>HYTFPKVWANSGTTADWQYVRRADNWQNNGFVDNVNSQQIRCFQSTHSPAQSTLSVAAGTTITYGAAPSVYHPGPMQFYLARVPDGQDINSWTGEGAVWFKIYHEQPTFGSQLTWSSNGKSSFPVKIPSCIKSGSYLLRAEHIGLHVAQSSGAAQFYISCAQLSITGGGSTEPGANYKVSFPGAYKASDPGILININYPVPTSYKNPGPSVFTC[2x]

An oxidative system was recently discovered in which extracellular flavocytochromes, that is, cellobiose dehydrogenases (CDHs), cooperate with copper-dependent lytic polysaccharide monooxygenases (LPMOs)8910111213 to catalyse redox-mediated glycosidic bond cleavage in crystalline cellulose, hemicelluloses and starch. CDHs are large flavocytochromes containing a haem b-binding cytochrome domain (CYT) connected by a long, flexible linker to a flavin adenine dinucleotide (FAD)-binding dehydrogenase domain (DH). The DH domain oxidizes cellobiose at the C1 position to cellobiono-1,5-lactone with reduction of FAD. The ensuing step involves inter-domain electron transfer (IET) from the reduced FAD to CYT haem b, presumably by single electron-transfer (ET) events, followed by ET from CYT to external electron acceptors such as LPMOs.

NcLPMO9F primarily attacks crystalline cellulose and promotes, in combination with cellulases, faster and more complete surface degradation. The structure of NcLPMO9F demonstrates that this LPMO shares the essential features of fungal LPMOs, including a β-sandwich fold and a catalytic surface-exposed copper centre in which the copper is coordinated by the ligands His1, His72 and Tyr157. We determined that NcLPMO9F is expressed in Pichia pastoris as a 214-residue non-glycosylated protein. As observed for the fungal LPMO GH61D from Phanerochaete chrysosporium, the N-terminal histidine in NcLPMO9F is not methylated, in contrast to the methylation of other N. crassa LPMOs expressed using the natural fungal host1523. Both NCS molecules in the NcLPMO9F crystal have copper ligated by four protein atoms in tetrahedral coordination and exhibit distorted octahedral coordination of the copper with mer-[MA3B3] geometry together with external ligands. In molecule A, two water molecules, one axial and one equatorial, satisfy the octahedral sphere. In molecule B, both water molecules are replaced by the carboxylate oxygen atoms of Asp33 from molecule A, which is similar to the coordination sphere observed in Streptomyces coelicolor ScLPMO10B where two oxygen atoms in an acetate molecule occupy the fourth equatorial and axial position on the solvent-facing side of Cu(II)34. These observations emphasize the possibility of the 4-coordinate Cu(II) in NcLPMO9F to accept one axial, and possibly also a fourth equatorial ligand (water or other). We observed very rapid NcCYT-to-NcLPMO9F ET with a haem b-kobs value of 67.2±2.3 s–1. Our results demonstrate unequivocally that, in the N. crassa CDH IIA-LPMO9F pair, the reduced haem b alone acts as the reductant of the NcLPMO9F copper centre in vitro.>AGRWNLEGCTALVTGGSRGIGYGIVEELASLGASVYTCSRNQKELNDCLTQWRSKGFKVEASVCDLSSRSERQELMNTVANHFHGKLNILVNNAGIVIYKEAKDYTVEDYSLIMSINFEAAYHLSVLAHPFLKASERGNVVFISSVSGALAV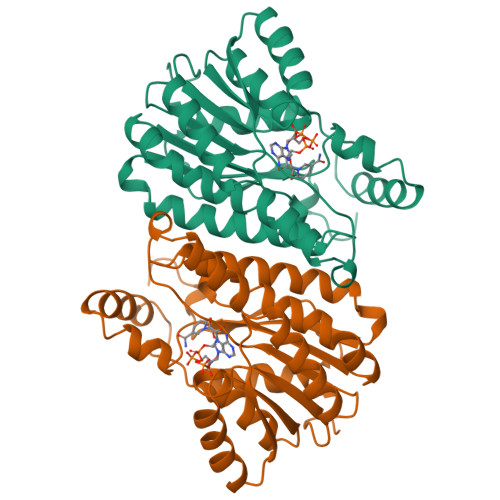PYEAVYGATKGAMDQLTRCLAFEWAKDNIRVNGVGPGVIATSLVEMTIQDPEQKENLNKLIDRCALRRMGEPKELAAMVAFLCFPAASYVTGQIIYVDGGLMANCGF[2x]>[2x]MSQPRTPEQALDTPGDCPPGRRDEDAGEGIQCSQRMLSFSDALLSIIATVMILPVTHTEISPEQQFDRSVQRLLATRIAVYLMTFLIVTVAWAAHTRLFQVVGKTDDTLALLNLACMMTITFLPYTFSLMVTFPDVPLGIFLFCVCVIAIGVVQALIVGYAFHFPHLLSPQIQRSAHRALYRRHVLGIVLQGPALCFAAAIFSLFFVPLSYLLMVTVILLPYVSKVTGWCRDRLLGHREPSAHPVEVFSFDLHEPLSKERVEAFSDGVYAIVATLLILDICEDNVPDPKDVKERFSGSLVAALSATGPRFLAYFGSFATVGLLWFAHHSLFLHVRKATRAMGLLNTLSLAFVGGLPLAYQQTSAFARQPRDELERVR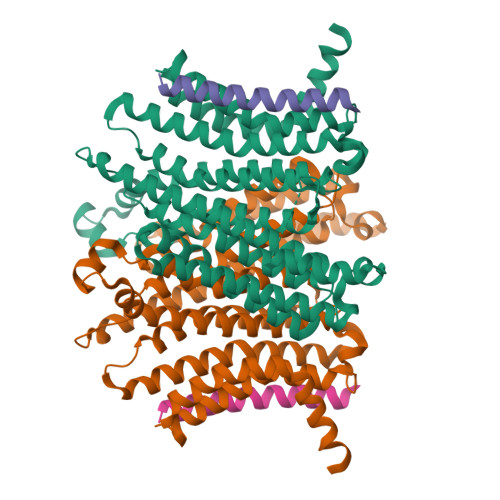VSCTIIFLASIFQLAMWTTALLHQAETLQPSVWFGGREHVLMFAKLALYPCASLLAFASTCLLSRFSVGIFHLMQIAVPCAFLLLRLLVGLALATLRVLRGLARPEHPPPAPTGQDDPQSQLLPAPC;>MAAPGSARRPLLLLLLLLLLGLMHCASAAMFMVKNGNGTACIMANFSAAFSVNYDTKSGPKNMTFDLPSDATVVLNRSSCGKENTSDPSLVIAFGRGHTLTLNFTRNATRYSVQLMSFVYNLSDTHLFPNASSKEIKTVESITDIRADIDKKYRCVSGTQVHMNNVTVTLHDATIQAYLSNSSFSRGETRCEQDRPSPTTAPPAPPSPSPSPVPKSPSVDKYNVSGTNGTCLLASMGLQLNLTYERKDNTTVTRLLNINPNKTSASGSCGAHLVTLELHSEGTTVLLFQFGMNASSSRFFLQGIQLNTILPDARDPAFKAANGSLRALQATVGNSYKCNAEEHVRVTKAFSVNIFKVWVQAFKVEGGQFGSVEECLLDENSMLIPIAVGGALAGLVLIVLIAYLVGRKRSHAGYQTI[2x]>[2x]MSLSYVKEGLAVLEDGRLIYITPEEFRQLLQGDAILAVYSKTCPHCHRDWPQLIQASKEVDVPIVMFIWGSLIGERELSA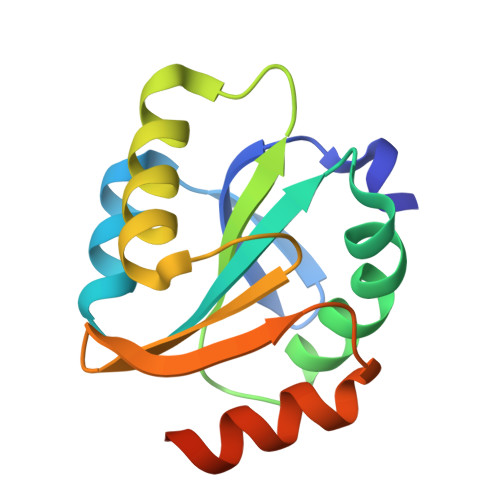ARLEMNKAGVEGTPTLVFYKEGRIVDKLVGATPWSLKVEKAREIYGGEGHHHHHH>[4x]MSNEIPKPVAPAPDILRCAYAELVVTDLAKSRNFYVDVLGLHVSYEDENQIYLRSFEEFIHHNLVLTKGPVAALKAMAFRVRTPEDVDKAEAYYQELGCRTERRKDGFVKGIGDALRVEDPLGFPYEFFFETTHVERLHMRYDLYSAGELV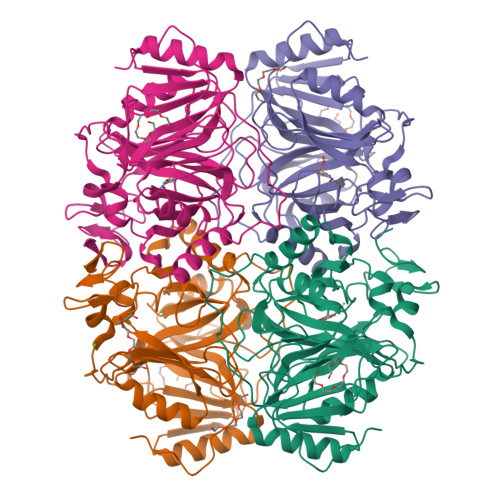RLDHFNQVTPDVPRGRKYLEDLGFRVTEDIQDDEGTTYAAWMHRKGTVHDTALTGGNGPRLHHVAFSTHEKHNIIQICDKMGALRISDRIERGPGRHGVSNAFYLFILDPDNHRIEIYTQDYYTGDPDNPTITWNVHDNQRRDWWGNPVVPSWYTEASKVLDLDGNVQEIIERTDDSELEVTIGADGFSFTRAGDEDGSYHGQASKGFKLGNQL> MTFAKIKFSAQIRLETGLHIGGSDAFAAIGAINSPVIKDPITNLPIIPGSSLKGKMRTLLAKVYNEKVAEKPSDDSDILSRLFGNSKDKRFKMGRLIFRDAFLSNADELDSLGVRSYTEVKFENTIDRITAEANPRQIERAIRNSTFDFE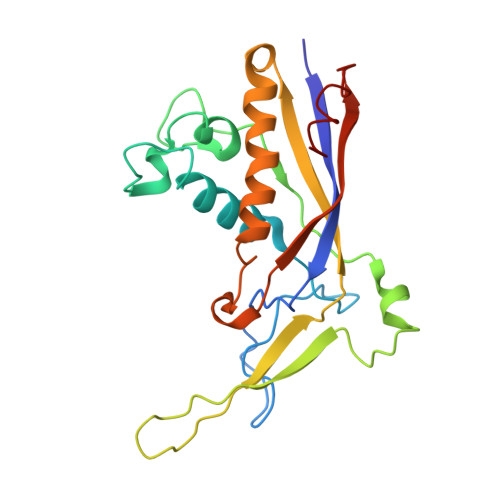LIYEITDENENQVEEDFKVIRDGLKLLELDYLGGSGSRGYGKVAFENLKATTVFGNYDVKTLNELLTAEV>MIDFGNFYSLIAKNHLSHWLETLPAQIANWQREQQHGLFKQWSNAVEFLPEIKPYRLDLLHSVTAESEEPLSAGQIKRIETLMRNLMPWRKGPFSLYGVNIDTEWRSDWKWDRVLPHLSDLTGRTILDVGCGSGYHMWRMIGAGAHLAVGIDPTQLFLCQFEAVRKLLGNDQRAHLLPLGIEQLPALKAFDTVFSMGVLYHRRSPLEHLWQLKDQLVNEGELVLETLVIDGDENTVLVPGDRYAQMRNVYFIPSALALKNWLKKCGFVDIRIADVSVTTTEEQRRTEWMVTESLADFLDPHDPGKTVEGYPAPKRAVLIARKP[2x]

Recently, we demonstrated that cmo5U modification requires the previously unknown metabolite carboxy-S-adenosine-L-methionine (Cx-SAM), which is generated by the CmoA-catalyzed conversion of prephenate and SAM to yield Cx-SAM and phenylpyruvate. Cx-SAM is subsequently utilized in the CmoB-catalyzed carboxymethylation of ho5U-containing tRNAs to yield the mature cmo5U-modified tRNAs, with no involvement of a mo5U intermediate. As predicted from sequence considerations, CmoB is composed of a Rossmann fold, coupled to a substrate-specific N-terminal domain of ∼100 residues that is unique to CmoB. Our biochemical, genetic and structural data demonstrate that the primary in vivo function of CmoB is as a carboxymethyl transferase in the biosynthesis of cmo5U-modified tRNAs.

Cx-SAM bound CmoB structures were determined in two crystal forms, resulting in 10 independent copies of the complex (two tetramers in one crystal form, and one dimer in the other), while the apo structure contains a single dimer in the asymmetric unit. The dimers exhibit symmetry-related interactions that recapitulate the expected tetramer. Continued refinement and modeling indicated that Cx-SAM is present at full occupancy and demonstrated similar atomic interactions in all 10 independent catalytic sites in both liganded structures. The side chains of Lys-91, Tyr-200 and Arg-315 interact with the carboxyl group of the S-carboxymethyl moiety of the Cx-SAM ligand. Three additional conserved residues within the CmoB family recognize the amino acid moiety of the ligand: the side chain of Lys-110 (815/818) forms polar interactions with the α-carboxy group, while the backbone carbonyl oxygen atoms of Gly-130 (817/818; the presence of a bulkier side chain would likely interfere with ligand binding) and Met-196 (606/818, where other instances are leucine) interact with the α-amino group of Cx-SAM. The side chain of Glu-182 (96% conservation) forms polar interactions with N6 of the adenine moiety and the side chain of Asp-152 (∼97% conserved in CmoB orthologs, and highly conserved in all members for SAM-dependent methyltransferase superfamily) interacts with the 2′- and 3′-hydroxyls. The side chain of Thr-154 (only 29.9% conservation) also forms a hydrogen bond with the 2′-hydroxyl of Cx-SAM. The Cx-SAM binding site is more exposed to solvent than observed for the Cx-SAM/SAM binding sites in CmoA and many other SAM-dependent methyltransferases, likely due to the need to accommodate bulky tRNA substrates. Considerable positive electrostatic potential surrounds the Cx-SAM binding pocket on the surface of the CmoB, consistent with the docking site of polyanionic tRNA molecules. In all subunits in both Cx-SAM bound structures, a feature modeled as a phosphate ion is present between two basic residues, Arg-202 and His-208 (98.3 and 67.1% conservation, respectively), with one of the presumed sulfate ions from the crystallization media present at a similar position in the apo structure.stearoyl adenylate | 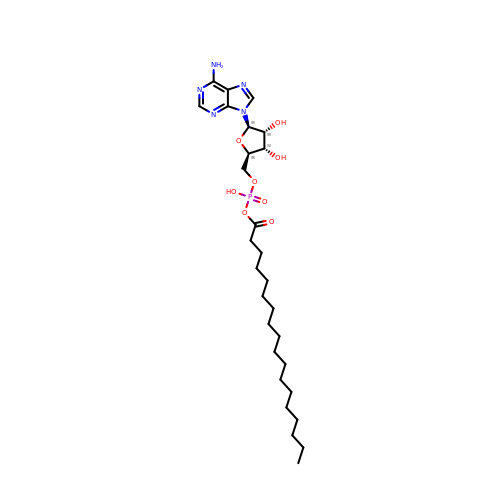C28 H48 N5 O8 P | SWOLRYFPKWBFHG-VGSCBBJJSA-N> MHHHHHHHHLVPRGSYDNREIVMKYIHYKLSQRGYEWDAGADVEENRTEAPEGTESEVVHKTLREAGDDFSRRYRRDFAEMSSQLHLTPFTARGRFATVVEELFRDGVNWGRIVAFFEFGGVMCVESVNREMSPL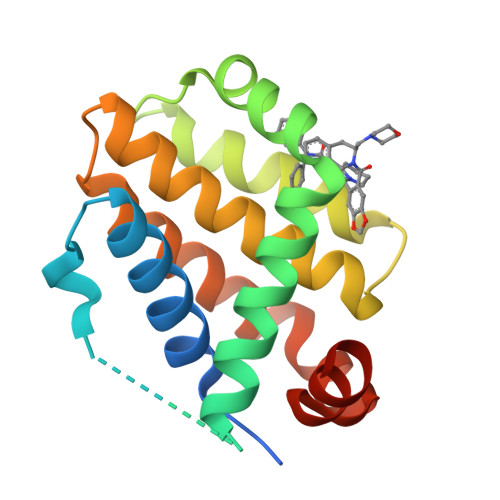VDNIALWMTEYLNRHLHTWIQDNGGWDAFVELYGPSM> MASDYKDDDDKGALEVLFQGPSSPMAGNLVSWACKLCRSPEGFGPISFYGDFTQCFIDGVILNLSAIFMITFGIRDLVNLCKKKHSGIKYRRNWIIVSRMALVLLEIAFVSLASLNISKEEAENFTIVSQYASTMLSLFVALALHWIEYDRSVVANTVLLFYWLFETFGNFAKLINILIRHTYEGIWYSGQTGFILTLFQVITCASILLLEALPKKPLMPHQHIHQTLTRRKPNPYDSANIFSRITFSWMSGLMKTGYEKYLVEADLYKLPRNFSSEELSQKLEKNWENELKQKSNPSLSWAICRTFGSKMLLAAFFKAIHDVLAFTQPQLLRILIKFVTDYNSERQDDHSSLQGFENNHPQKLPIVRGFLIAFAMFLVGFTQTSVLHQYFLNVFNTGMYIKSALTALIYQKSLVLSNEASGLSSTGDIVNLMSVDVQKLQDLTQWLNLIWSGPFQIIICLYSLYKLLGNSMWVGVIILVIMMPLNSFLMRIQKKLQKSQMKYKDERTRVISEILNNIKSLKLYAWEKPYREKLEEVRNNKELKNLTKLGCYMAVTSFQFNIVPFLVSCCTFAVFVYTEDRALTTDLVFPALTLFNLLSFPLMIIPMVLNSFIEASVSIGRLFTFFTNEELQPDSVQRLPKVKNIGDVAINIGDDATFLWQRKPEYKVALKNINFQAKKGNLTCIVGKVGSGKTALLSCMLGDLFRVKGFATVHGSVAYVSQVPWIMNGTVKENILFGHRYDAEFYEKTIKACALTIDLAILMDGDKTLVGEKGISLSGGQKARLSLARAVYARADTYLLDDPLAAVDEHVARHLIEHVLGPNGLLHTKTKVLATNKVSALSIADSIALLDNGEITQQGTYDEITKDADSPLWKLLNNYGKKNNGKSNEFGDSSESSVRESSIPVEGELEQLQKLNDLDFGNSDAISLRRASDATLGSIDFGDDENIAKREHREQGKVKWNIYLEYAKACNPKSVCVFILFIVISMFLSVMGNVWLKHWSEVNSRYGSNPNAARYLAIYFALGIGSALATLIQTIVLWVFCTIHASKYLHNLMTNSVLRAPMTFFETTPIGRILNRFSNDIYKVDALLGRTFSQFFVNA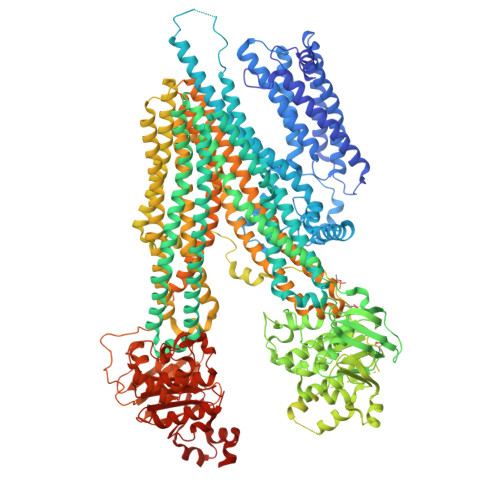VKVTFTITVICATTWQFIFIIIPLSVFYIYYQQYYLRTSRELRRLDSITRSPIYSHFQETLGGLATVRGYSQQKRFSHINQCRIDNNMSAFYPSINANRWLAYRLELIGSIIILGAATLSVFRLKQGTLTAGMVGLSLSYALQITQTLNWIVRMTVEVETNIVSVERIKEYADLKSEAPLIVEGHRPPKEWPSQGDIKFNNYSTRYRPELDLVLKHINIHIKPNEKVGIVGRTGAGKSSLTLALFRMIEASEGNIVIDNIAINEIGLYDLRHKLSIIPQDSQVFEGTVRENIDPINQYTDEAIWRALELSHLKEHVLSMSNDGLDAQLTEGGGNLSVGQRQLLCLARAMLVPSKILVLDQATAAVDVETDKVVQETIRTAFKDRTILTIAHRLNTIMDSDRIIVLDNGKVAEFDSPGQLLSDNKSLFYSLCMEAGLVNENGLVPRGSSAHHHHHHHHH> MHHHHHHGEASPVDPLRPVVDASIQPLLKEHRIPGMAVAVLKDGKAHYFNYGVANRESGAGVSEQTLFEIGSVSKTLTATLGAYAVVKGAMQLDDKASRHAPWLKGSAFDSITMGELATYSAGGLPLQFPEEVDSSEKMRAYYRQWAPVYSPGSHRQYSNPSIGLFGHLAASSLKQPFAPLMEQTLLPGLGMHHTYVNVPKQAMASYAYGYSKEDKPIRVNPGMLADEAYGIKTSSADLLRFVKANIGGVDDKALQQAISLTHQGHYSVGGMTQGLGWESYAYPVTEQTLLAGNSAKVILEANPTAAPRESGSQVLF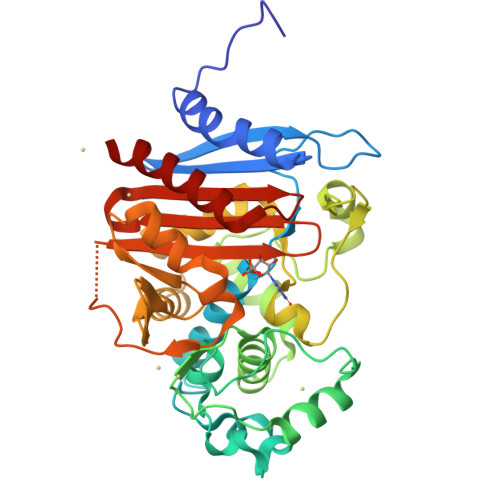NKTGSTNGFGAYVAFVPARGIGIVMLANRNYPIEARIKAAHAILAQLAG> MKKYLLSFLLSMIL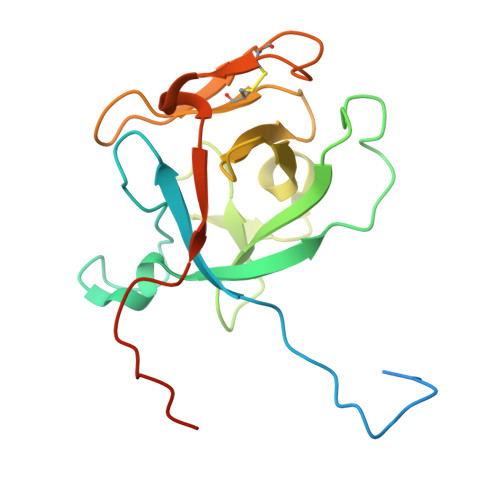TLTSHAESNPDPTTYPDVELSPPPRISLRSLLTAQPIKNDHYDSHNYLSTHWELIDYKGKEYEKLRDGGTLVQFKVVGAAKCFAFPGEGTTDCKDIDHTVFNLIPTNTGAFLIKDALLGFCMTSHDFDDLRLEPCGISVSGRTFSLAYQWGILPPFGPSKILRPPVGRNQGS> MSNHHHHHHHHHHENLYFQSMSGFLIPNAKFTSNNGFEFLLPYYWNIAPNFDATITPHYMERRGLQWQNEFRYLLAPGSGTMALDWLPNDRIYTGPDGTDKNATRWLYYWGHSGVMDQVWRFNINYTRVSDPAYFTDLTSQYGSTTDGYATQIFTAGYANENWNATLSSKQFQVFTAAGNSNAYRAQPQLDMNYYKNDVGPFDMHVYGQAAKFTSVNPTNPEASRFHIEPTVNLPLSNSWGSINTEAKLLATHYQQDIPASFADNASNPKLKDSVNRVLPQFKVDGKVVFDRSMDWATGFTQTLEPRAQYLYVPYRNQDDIYIYDTTLMQSDYSGLFRDRTYSGLDRIASANQVSTGLTSRIYDDARVERFNVSVGQIYYFSRSRTGNTEAIDNSNATGSLVWAGDTFWRINDQLGLKGGAQYDTRLGSLTLGNAIMEYRKDADRMIQLNYRYASPKYIQAAVPKVYNPDYQQGISQVGTTASWPIADRWAIVGAYYYDTKAKQPASQLVGLQYNTCCWAVNLGYERKITGWNAQGQTSKYDNKIGFNIELRGLSGGHSLGTAQMLNSGI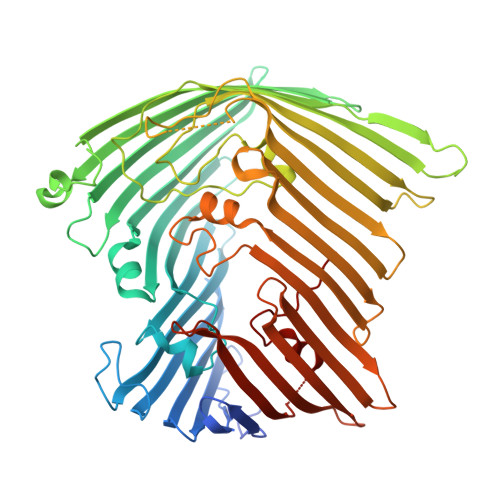LPYQSAF> GSLELELQNLELLVHIAEVLARLARRTGNEEALEHAARVAEEVAKQAEEIAREARYRGDLRLALEALRIMVEAARVLAEIARERGNEELLQKAEELAREALRQVREISKRLQEEGNIELALKANRLLIDALEVLVRIMRHR;> SSLEEKIEELVKELIKHTEELRRLLEKLVKEGGASEEYLLELLENLVRLARVIAEVAREQGNEELLEEAARLAEEAARQAEELAREARYEGDLELALKALQILVNAARVLAEIARDRGNEELLQKAAELAKEAARQAEEIAKEARERGNFELALEALEILNEAARVLARIAHHRGNQELLEEAWRLTHRSAKWSREIAEQARKEGE;> SPRLVLRALENMVRAAHTLAEIARDNGNEEWLERAARLAEEVAR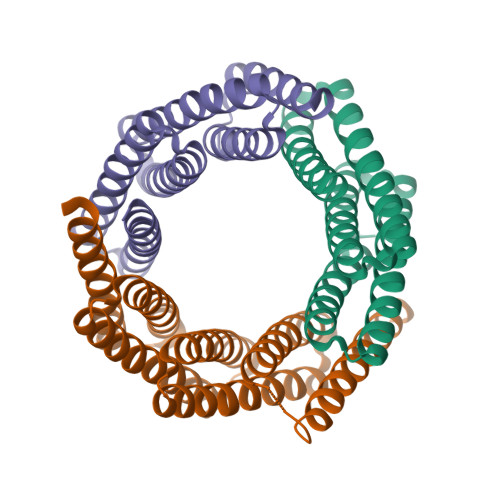RAEELAREAREKGDLELALKALQILVNAAYVLAEIARDRGNEELLKKAHELARKAAEEAQKIAEQARYEGNLELFNKALRILLEAIRVLIEHDDSEEAARELIRRLEELLEQSRRSMKG> PSSSMADFRKFFAKAKHIVIISGAGVSAESGVPTFRGAGGYWRKWQAQDLATPLAFAHNPSRVWEFYHYRREVMGSKEPNAGHRAIAECETRLGKQGRRVVVITQNIDELHRKAGTKNLLEIHGSLFKTRCTSCGVVAENYKSPICPALSGKGAPEPGTQDASIP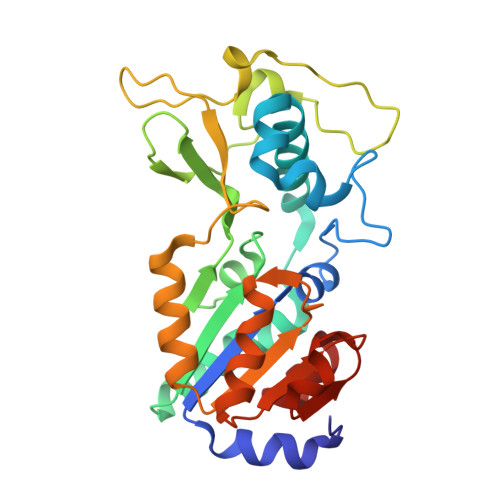VEKLPRCEEAGCGGLLRPHVVWFGENLDPAILEEVDRELAHCDLCLVVGTSSVVYPAAMFAPQVAARGVPVAEFNTETTPATNRFRFHFQGPCGTTLPEALA>GSGNSHTTPWTNPGLAENF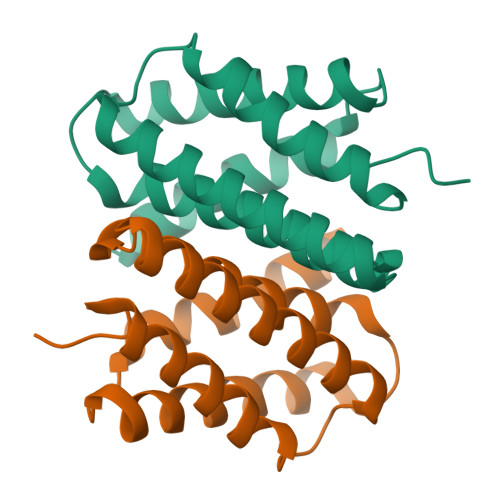MNSFMQGLSSMPGFTASQLDDMSTIAQSMVQSIQSLAAQGRASPNKLQALNMAFASSMAEIAASEEGGGSLSTKTSSIASAMSNAFLQTTGVVNQPFINEITQLVSMFAQAGMNDVSA[6x]>[2x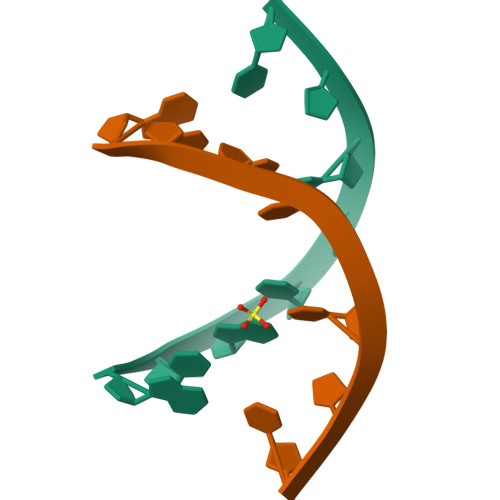]GXGTACAC>[10x]MGLH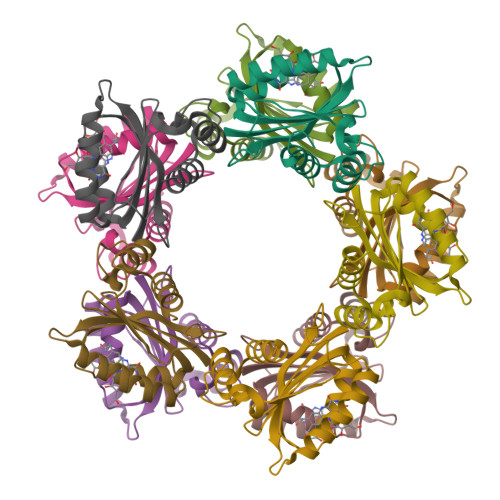RLIYLSCATDGLSYPDLRDIMAKSEVNNLRDGITGMLCYGNGMFLQTLEGDRQKVSETYARILKDPRHHSAEIVEFKAIEERTFINWSMRLVQLGEMDSDTIRRLRLKYSPAATFQPRSMTAEQCFRFLKELYDMSQGS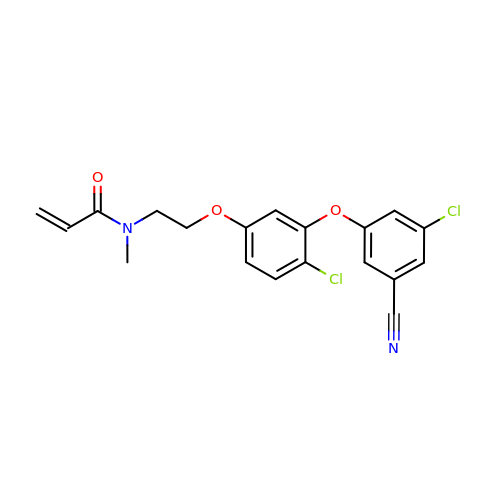N-{2-[4-chloro-3-(3-chloro-5-cyanophenoxy)phenoxy]ethyl}-N-methylprop-2-enamide | C19 H16 Cl2 N2 O3 | MYJVBQAXXKBPNA-UHFFFAOYSA-N>[2x]YTPVAVQCQEAQLVVTVHRDLFGTGRLINAADLTLGPAACKHSSLNAAHNTVTFAAGLHECGSVVQVTPDTLIYRTLINYDPSPASNPVIIRTNPAVIPIECHYPRREQVSSNAIRPTWSPFNSALSAEERLVFSLRLMSDDWSTERPFTGFQLGDILNIQAEVSTENHVPLRLFVDSCVAALSPD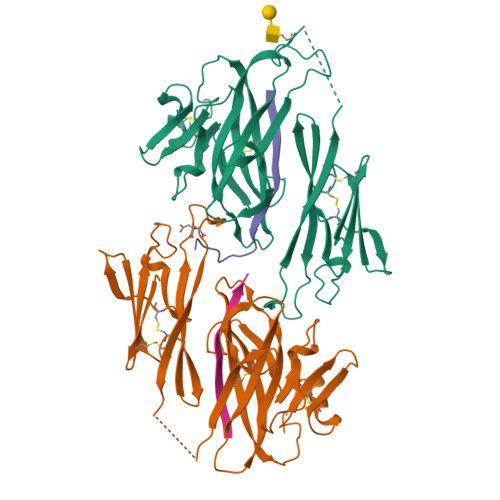GDSSPHYAIIDFNGCLVDGRVDDTSSAFITPRPREDVLRFRIDVFRFAGDNRNLIYITCHLKVTPADQGPDPQNKACSFNKARNTWVPVEGSRDVCNCCETGNCEPPALSR;>AFAADAGKEVAADVVIGPVLLSADHHHHHH[2x]> AMGNDTYQPINCDDYDNLELACQHHLMLTLELKDGE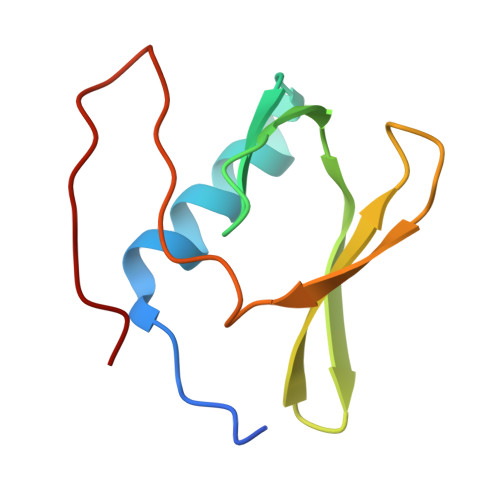KLQAKASDLVSRKNVEYLVVEAAGETRELRLDKITSFSHPEIGTVVVSES>MNTKYNKEFLLYLAGFVDGDGSI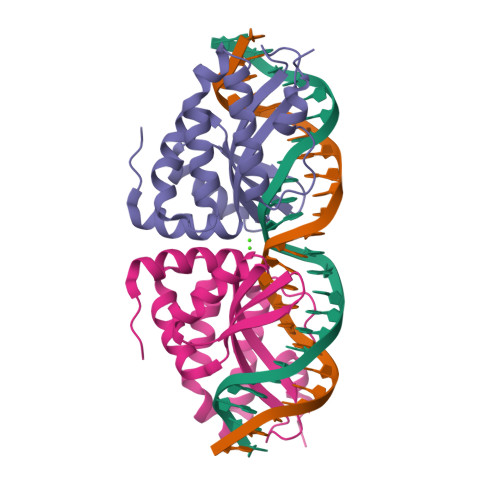IAQIRPNQSYKFKHQLSLTFQVTQKTQRRWFLDKLVDEIGVGYVRDRGSVSDYILSEIKPLHNFLTQLQPFLKLKQKQANLVLKIIEQLPSAKESPDKFLEVCTWVDQIAALNDSKTRKTTSETVRAVLD[2x]Overcoming lysogenization defect (OLD) proteins constitute a family of uncharacterized nucleases present in bacteria, archaea, and some viruses. These enzymes contain an N-terminal ATPase domain and a C-terminal Toprim domain common amongst replication, recombination, and repair proteins. Here we identify and define two classes of OLD proteins based on differences in gene neighborhood and amino acid sequence conservation and present the crystal structures of the catalytic C-terminal regions from the Burkholderia pseudomallei and Xanthamonas campestris p.v. campestris Class 2 OLD proteins at 2.24 Å and 1.86 Å resolution respectively. The structures reveal a two-domain architecture containing a Toprim domain with altered architecture and a unique helical domain.

The truncated XccCTR construct, in contrast, yielded crystals that routinely diffracted beyond 2 Å and three independent structures were solved using SAD datasets from platinum, mercury, and iodide derivatives. These models show strong agreement with an overall RMSD of 0.42–0.44 Å and display only slight deviations at the N-terminus near the mercury-binding site and within a flexible loop containing two adjacent glycines (G479 and G480). Residues 374–387 and 458–463 are disordered in each structure, though present in the purified construct. The XccCTR derivative structures contain nothing in their active sites. Similar interactions are observed between the domains in the XccCTR. The position of these helices is consistent between the BpCTR and XccCTR structures, arguing it is an intrinsic topological feature and not simply due to crystal packing. In contrast, truncated constructs containing the C-terminal region of each homolog (XccCTR, BpCTR) were each monomeric by SEC-MALS analysis. XccFL and XccCTR similarly can degrade DNA with Mg2+and Mn2+ but also are partially active in Zn2+.

> RDEEDLQRYIDVTRGEIFFSRGVILVEGDAERFIVPAFAEVLNIPLDMLGITVCSVGGTNFTPYVKLLGPEGLNIPHVILTDRDPTNGNHPLVRRRLINVLDVIEGGVDHEELDADEVIKLAEQYGYFVNENTLEPELFAGGLAEDMQEVIREELPRLRRETLNALQQWVDDPAQIDEDLLLRLIERIGKGRFAQALAPSVSEDVCPAYIRSALEHIRDAIALEHHHHHH> MYRVAVIPGDGIGPEVIDGAVRVLKAVTGRVRFEYYEGGVDVFQECGSPIRE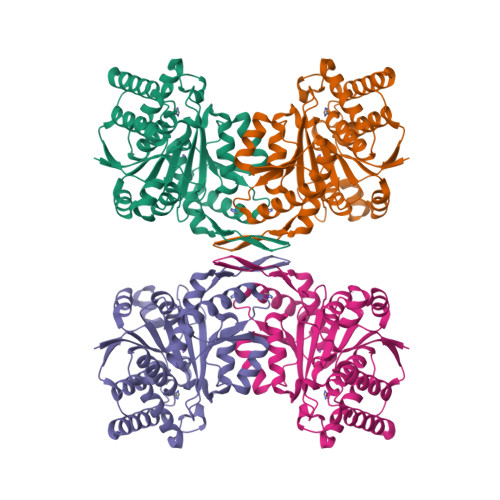EDLEEIRRSDAVLFGATTTPFDLPGYRSLILTLRKELGLYANLRIIPDLRTGREIVIVRENSEGLYFGIGAVVNGRAVDVRLITREGAERIARFAVEQAKARGSFITFVHKANVLTGDKFFRRIVREVAGEEGVEVRDAIIDSFTIKLVRNPWEHGVILSENLFGDILSDLATVHAGSIGIVPSGNYGDGIALFEPVHGSAPDIAGKGIANPIGAILSGAMLLDYLGLDGSLIRAAVRGYVVNGELTPDMGGRARTEDVVRGIIGEIEDLLSMDEVWRDEIRLSRLESDISRMAGHHHHHH Lipoxygenases (LOX) are key enzymes in the initial step of lipid-mediator biosynthesis. They catalyze a regio- and stereo specific dioxygenation of polyunsaturated fatty acids to yield fatty acid hydroperoxides, which can be further metabolized to a variety of signaling molecules with diverse biological functions. CspLOX2 is the LOX with the highest relative amount of bis-allylic product reported so far, hence it is a suitable candidate to study the molecular basis of the dioxygen positioning at the bis-allylic position. We demonstrate the importance of an active site clamp around the pentadiene system, which fixes the pentadiene during the reaction resulting in 11-HPODE formation.

A key residue that is located opposite of the iron ion and hence likely restricts the space in the kink region is the highly conserved Leu304. In general, mutations inserted close to the iron in the kink of the channel had the strongest effects on the product specificity, while amino acid substitutions closer to the entrance or the bottom of the channel resulted in smaller changes. In case of 13-HPODE, Leu304 and Leu502 are rather facing the side of 13S-HPODE formation, while Leu506 faces the side for 13R-HPODE formation.

>[2x]MVQPSLPQDDTPDQQEQRNRAIAQQREAYQYSETAGILLIKTLPQSEMFSLKYLIERDKGLVSLIANTLASNIENIFDPFDKLEDFEEMFPLLPKPLVMNTFRNDRVFARQRIAGPNPMVIERVVDKLPDNFPVTDAMFQKIMFTKKTLAEAIAQGKLFITNYKGLAELSPGRYEYQKNGTLVQKTKTIAAPLVLYAWKPEGFGDYRGSLAPIAIQINQQPDPITNPIYTPRDGKHWFIAKIFAQMADGNCHEAISHLARTHLILEPFVLATANELAPNHPLSVLLKPHFQFTLAINELAREQFISAGGYADDLLAGTLEASIAVIKAAIKEYMDNFTEFALPRELARRGVGIGDVDQRGENFLPDYPYRDDAMLLWNAIEVYVRDYLSLYYQSPVQIRQDTELQNWVRRLVSPEGGRVTGLVSNGELNTIEALVAIATQVIFVSGPQHAAVNYPQYDYMAFIPNMPLATYATPPNKESNISEATILNILPPQKLAARQLELMRTLCVFYPNRLGYPDTEFVDVRAQQVLHQFQERLQEIEQRIVLCNEKRLEPYTYLLPSNVPNSTSI>MMSEIIAVANQKGGVGKTTTAVNLAASLAVHEKKILLIDFAPQANATSSLGFRRDKIDYDIYHVLIGRKQISQVILKTQMPFLDLVPSNLGLAGFEKTFYDSQDENKRGELMLKNALESVVGLYDYIIIDSPPALGPLTINSLSAAHSVIIPIQCEFFALEGTKLLLNTIRMLQKSTNPKLKIRGFLPTMHVPQLNLTKGVLAELFKYFDSEFFRDSATGEYIMIPKSVKLAESPSFGKPILLYDIKSNGSIAYQKLAQSILQG[2x]

The ParABS system, composed of ParA (an ATPase), ParB (a DNA binding protein), and parS (a centromere-like DNA), regulates bacterial chromosome partition. In Helicobacter pylori, ParA and ParB homologs are encoded as HpSoj and HpSpo0J (HpParA and HpParB), respectively. ParA forms as a dimer in the ATP-bound state that can bind to nsDNA through a continuous basic binding patch formed by arginine/lysine residues. The partition complex interacts with the nucleoid-bound ParA forming the nucleoprotein ParA–ParB–DNA complex, known as the nucleoid–adaptor complex (NAC).

A key residue, aspartic acid (D41 in HpParA), coordinates the water nucleophile (WNu) and initiates ATP hydrolysis, playing a significant role in ParA ATP-hydrolysis. To investigate the relationship between WNu and ATP hydrolysis, we solved the crystal structure of HpParAD41A in complex with ATP, HpParAD41A-ATP. The overall structure of the HpParAD41A is similar to that of the HpParA, with a root mean square deviation (r.m.s.d.) of 0.4 Å (in Cα). In the ATP binding pocket, the electron density map of the γ-phosphate of ATP clearly revealed a complete and unhydrolyzed ATP molecule. We can clearly observe the WNu located and coordinated between the γ-phosphate and Asp41 in the wild type, while the WNu cannot be observed in the HpParAD41A-ATP. This suggests that Asp41 likely captures the essential WNu and plays a crucial role in initiating ATP hydrolysis. As a result, HpParAD41A exhibits reduced ATP hydrolysis activity and functions as a deficient mutant in ATP hydrolysis. HpParAD41A is an ATP hydrolysis deficient mutant with lower ATP hydrolysis (0.4 ± 0.2 mol Pi released/mole HpParAD41A·hour−1) compared to HpParA wild type (1.0 ± 0.3 moles Pi released/mole HpParA·hour−1). We observed that HpParAD41A has a tendency to prolong the ATP-bound state when in dimer form.> MAHAGRTGYDNREIVMKYIHYKLSQRGYEWDA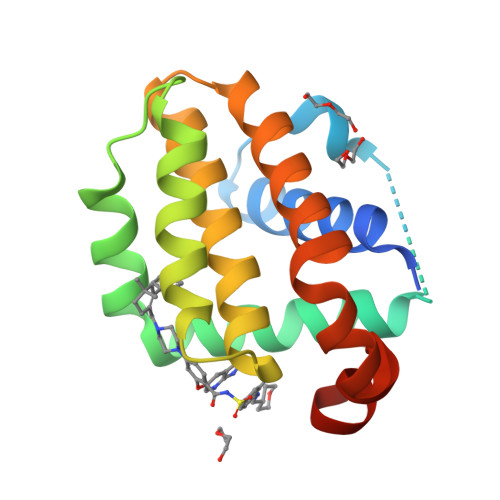GDDVEENRTEAPEGTESEVVHLTLRQAADDFSRRYRRDFAEMSSQLHLTPFTARGRFATVVEELFRDGVNWGRIVAFFEFGGVMCVESVNREMSPLVDNIALWMTEYLNRHLHTWIQDNGGWDAFVELYGPSMR> GTGDGSELPKEMEEYFEMLQREIDKAYEIAKKARAQGKDPSLDVEIPQATDMAGRVESLVGPPGVAKRIRELVKEYGKEIAALKIVDEIIEGKFGDLGSREKYAEQAVRTALAILTEGIVSAPIEGIANVKIKRNTWADNSEYLALYYAGPIRSSGGTAQALSVLVGDYVRRKLGLDRFKPSEKHIERMVEEVDLYHRAVTRLQYHPSPEEVRLAMRNIPIEITGEATDDVEVSHRDVPGVETNQLRGGAILVLAEGVLQKAKKLVKYIDKMGIEGWEWLKEFVEAKEKGEPKEEGKEESLAESTLEETKVEVDMGFYYSLYQKFKEEIAPSDKYAKEVIGGRPLFSDPSKPGGFRLRYGRSRASGFATWGINPATMILVDEFLAIGTQLKTERPGKGAVVTPVTTIEGPIVKLKDGSVLRVDDYNLALKVREDVEEILYLGDAVIAFGDFVENNQTLLPANYCEEWWILEFVKALKEIYEVHLEPFTENEEESIEEASDYLEIDPEFLKEMLRDPLRVKPPVELAIHFSEVLGIPLHPY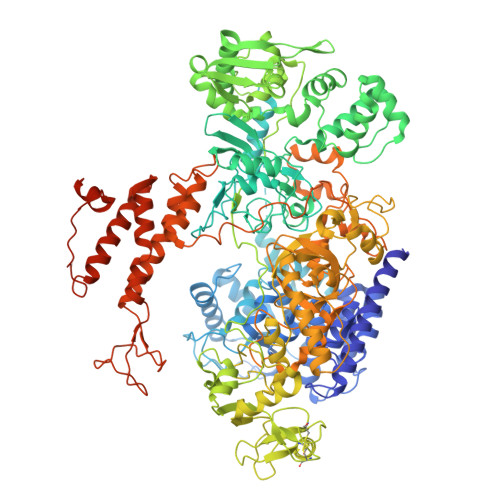YTLYWNSVEPKDVEKLWRLLKNYAEIEWSNFRGIKFAKKIVISQEKLGDSKRTLELLGLPHTVRDGNVIVDYPWAAALLTPLGNLNWEFMAKPLYATIDIINENNEIKLRDRGISWIGARMGRPEKAKERKMKPPVQVLFPIGLAGGSSRDIKKAAEEGKVAEVEIAFFKCPKCGHVGPEHLCPNCGTRKELLWVCPRCNAEYPESQAEGYNYTCPKCNVKLRPYAKRKIRPSELLNRAMENVKVYGVDKLKGVMGMTSGWKMPEPLEKGLLRAKNDVYVFKDGTIRFDATDAPITHFRPREIGVSVEKLRELGYTHDFEGKPLVSEDQIVELKPQDIILSKEAGRYLLKVAKFVDDLLEKFYGLPRFYNAEKMEDLIGHLVIGLAPHTSAGIVGRIIGFVDALVGYAHPYFHAAKRRNCDGDEDAVMLLLDALLNFSRYYLPEKRGGKMDAPLVITTRLDPREVDSEVHNMDIVRYYPLEFYEATYELKSPKELVGVIERVEDRLGKPEMYYGLKFTHDTDDIALGPKMSLYKQLGDMEEKVRRQLEVAKRIRAVDEHGVAEKILNSHLIPDLRGNLRSFTRQEFRCVKCNTKFRRPPLNGKCPVCGGKIVLTVSKGAIEKYLGTAKMLVTEYNVKNYTRQRICLTERDIDSLFENVFPETQLTLIVNPNDICQRLVMARTGEVNKSGLLENLSNGSKKTEKAEKAEKPRKKSDEKPKKKRVISLEEFFSRKSK>FQSNAMAKSEGKVNGATLMARALQQQGVQYMFGIVGFPVIPIAIAAQREGITYIGMRNEQSASYAAQAASYLTGRPQACLVVSGPGVVHALAGLANAQVNCWPMLLIGGASAIEQNGMGAFQEERQVLLASPLCKYAHQVERPERIPYYVEQAVRSALFGRPGAAYLDMPDDVILGEVEEAAVRPAATVGEPPRSLAPQENIEAALDALQSAKRPLVIVGKGMAWSRAENEVRQFIERTRLPFLATPMGKGVMPDDHPLSVGGARSHALQEADLVFLLGARFNWILHFGLPPRYSKDVRVIQLDLSAEEIGNNRQAEVALVGDGKAIVGQLNQALSSRQWFYPAETPWREAIAAKIAGNQAAVAPMIADNTSPMNYYRVYRDIAARLPRNAIIVGEGANTMDIGRTQMPNFEPRSRLDAGSYGTMGIGLGFAVAAAAVHPGRPVIAVQGDSAFGFSGMEFETAARYGMPIKVIILNNGGIGMGSPAPRDGQPGMPHALSHDARYERIAEAFGGAGFYVTDSAELGPALDAAMAFKGPAIVNIKIAATADRKPQQFNWHG[4x]

One such enzyme is 2-hydroxyacyl-CoA lyase/synthase (HACL/S), which catalyzes the reversible cleavage of 2-hydroxyacyl-CoA (2hcCoA) into formyl-CoA (fCoA) and an aldehyde or ketone. Originally identified in the mammalian α-oxidation pathway of 3-methyl-branched fatty acids, HACL/S has demonstrated remarkable catalytic reversibility, as it is capable of condensing fCoA with various substrates covering a wide range of aldehydes and ketones with different carbon chain lengths. All the enzymes are tetramers, specifically dimers of dimers (α2), where α2 dimer represents a catalytical unit. The three domains have specific functions: the N-terminal domain binds the pyrimidine of ThDP (PYR), the middle domain has a regulatory function (R) and binds ADP, and the C-terminal domain binds the pyrophosphoryl group (PP) of ThDP.

In all ApbHACL/S structures, the whole tetramer is in the asymmetric unit. The monomers are structurally very similar to each other, with root mean square deviation (RMSD) on superimposed Cα positions in the range of 0.2–0.4 Å but locally show distinct conformations. Therefore, there are four different representations of the active sites formed by four slightly altered protomers in the tetramer. A similar intermediate ThDP-hmCoA is also found in the structure of ApbHACL/S-CoA. In these two structures ApbHACACL/S-CoA and ApbHACL/S-fCoA, the distances between C2 of ThDP and C1 of hmCoA are significantly longer than a regular C–C bond (1.54 Å) with 1.8 and 1.9 Å, respectively. Additionally, the C1-O distance in ApbHACL/S-CoA is 1.4 Å which is close to that of a regular hydroxymethyl but 2.0 Å for the same distance in ApbHACL/S-fCoA is much elongated. This suggests that these two intermediates found in these structures represent slightly different reaction states. The structures of ApbHACL/S with CoA and fCoA trapped intermediate states serve as examples. Structures of both TbHACL/S and ApbHACL/S with and without acyl-CoA indicate that there is no notable difference in main chains and side chains except for the well-ordered C-terminal regions.>[8x]GMSQATAKVNREVQAFLQDLKGKTIDHVFFVACGGSSAIMYPSKYVFDRESKSINSDLYSANEFIQRNPVQLGEKSLVILCSHSGNTPETVKAAAFARGKGALTIAMTFKPESPLAQEAQYVAQYDWGDEALAINTNYGVLYQIVFGTLQVLENNTKFEQA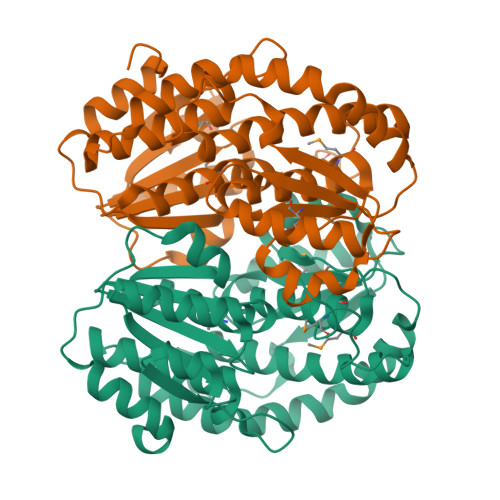IEGLDQLQAVYEKALKQEADNAKQFAKAHEKESIIYTMASGANYGVAYSYSICILMEMQWIHSHAIHAGEYFHGPFEIIDESVPFIILLGLDETRPLEERALTFSKKYGKKLTVLDAASYDFTAIDDSVKGYLAPLVLNRVLRSYADELAEERNHPLSHRRYMWKVEY> ASSPANKVYQDRFESMYSKIKDPANGYFSEQGIPYHSIETLMVEAPDYGHVTTSQAMSYYMWLEAMHGRFSGDFTGFDKSWSVTEQYLIPTEKDQPNTSMSRYDANKPATYAPEFQDPSKYPSPLDTSQPVGRDPINSQLTSAYGTSMLYGMHWILDVDNWYGFGARADGTSKPSYINTFQRGEQESTWETIPQPCWDEHKFGGQYGFLDLFTKDTGTPAKQFKYTNAPDADARAVQATYWADQWAKEQGKSVSTSVGKATKMGDYLRYSFFDKYFRKIGQPSQAGTGYDAAHYLLSWYYAWGGGIDSTWSWIIGSSHNHFGYQNPFAAWVLSTDANFKPKSSNGASDWAKSLDRQLEFYQWLQSAEGAIAGGATNSWNGRYEAVPSGTSTFYGMGYVENPVYADPGSNTWFGMQVWSMQRVAELYYKTGDARAKKLLDKWAKWINGEIKFNADGTFQIPSTIDWEGQPDT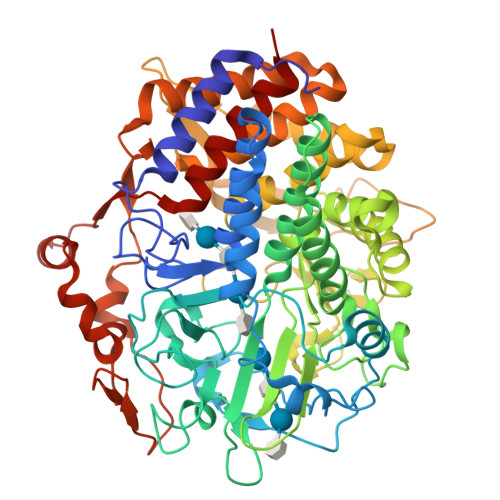WNPTQGYTGNANLHVKVVNYGTDLGCASSLANTLTYYAAKSGDETSRQNAQKLLDAMWNNYSDSKGISTVEQRGDYHRFLDQEVFVPAGWTGKMPNGDVIKSGVKFIDIRSKYKQDPEWQTMVAALQAGQVPTQRLHRFWAQSEFAVANGVYAILFPD> SPRLVLRALENMVRAAHTLAEIARDNGNEEWLERAARLAEEVARRAEELAREAREKGDLELALKALQILVNAAYVLAEIARDRGNEELLKKAHELAR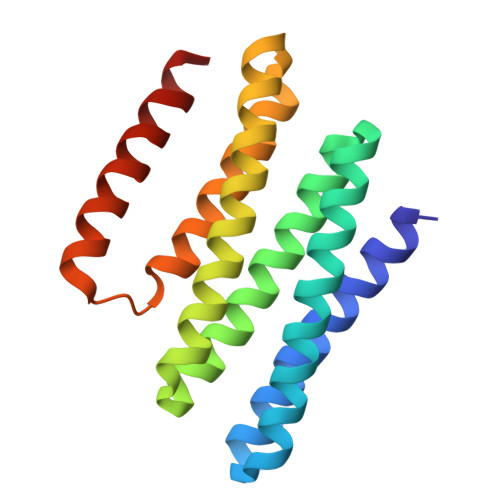KAAEEAQKIAEQARYEGNLELFNKALRILLEAIRVLIEHDDSEEAARELIRRLEELLEQSRRSMKG>GPHMEVGTVVQEEMKFR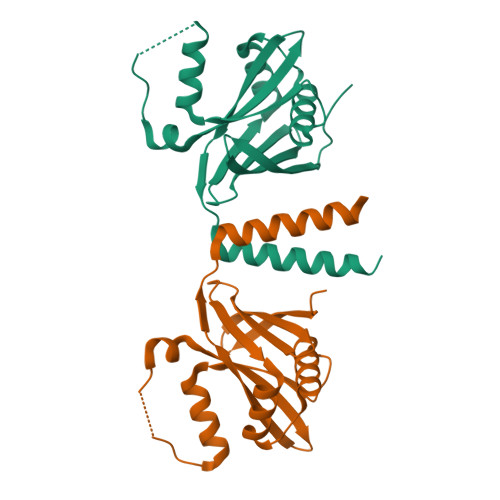GSEFAVKVEMAERLLIVEISDVVTADQWRGEFGPAYIEDLTRKTGNFKQFPVFCSMLESAVHKSSDSVTLDLLTYSDLELLRNRKAGVVGRPRAQPQSPALSAKRYLILIYTVEEARIHYPLPLPYLGKPDPAELQKEIRALRSELKTLGLRGD[2x]>MVPGACPLILRLSPTLHSADLIRDIDAMRWFLFEDTGVPLPEVNIEVLPEPTEKLTVLLYQEPVFSLSIPAQADYLLIGADASVVGDSQTLPNGMGQICWLTKDMAHKAQGFGLDVFAGSQRISALLKCVLLRHMGEFIGVQE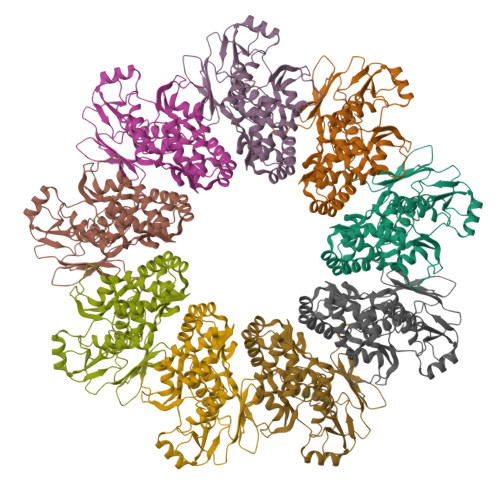TRYLMNAMEKNYSELVKELQRQLPINKIAETLQRLVSERVSIRDLRLIFGTLIDWAPREKDVLMLTEYVRIALRRHILRRLNPEGKPLPILRIGEGIENLVRESIRQTAMGTYTALSSRHKTQILQLIEQALKQSAKLFIVTSVDTRRFLRKITEATLFDVPILSWQELGEESLIQVVESIDLSEEELADNEE[9x]> MKKFLPGLLLMGLV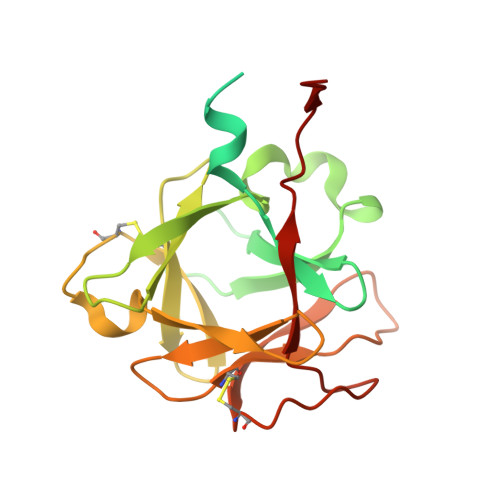ACSSNQRMSDYSQPESQSDLAPKSSTTQFQPQPLLSKASSMPLNLLSSSKNGQVSPSEPSNFMTLMGQNGALLTVWALAKRNWLWAYPNIYSQDFGNIRNWKIEPGKHREYFRFVNQSLGTCIEAYGNGLIHDTCSLDKLAQEFELLPTDSGAVVIKSVSQGRCVTYNPVSPTYYSTVTLSTCDGATEPLRDQTWYLAPPVLEATAVN>[2x]HRKDHFIVCGHSILAINTILQLNQRGQNVTVISNLPEDDIKQLEQRLGDNADVIPGDSNDSSVLKKAGIDRCRAILALSDNDADNAFVVLS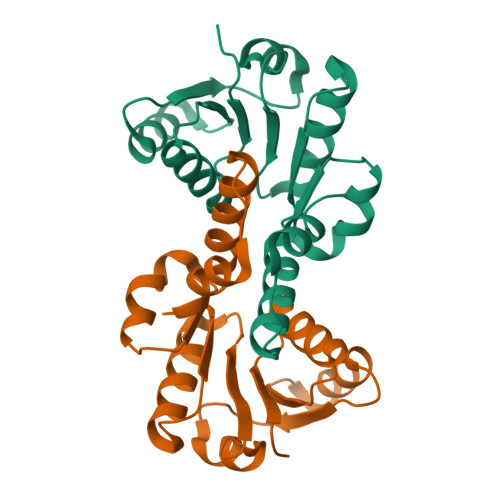AKDMSSDVKTVLAVSDSKNLNKIKMVHPDIILSPQLFGSEILARVLNGEEINNDMLVSMLLN(S)-7-((R)-sec-butoxy)-1-(4-chlorophenyl)-6-methoxy-2-(4-(methyl(pyridin-4-ylmethyl)amino)phenyl)-1,2-dihydroisoquinolin-3(4H)-one | C33 H34 Cl N3 O3 | 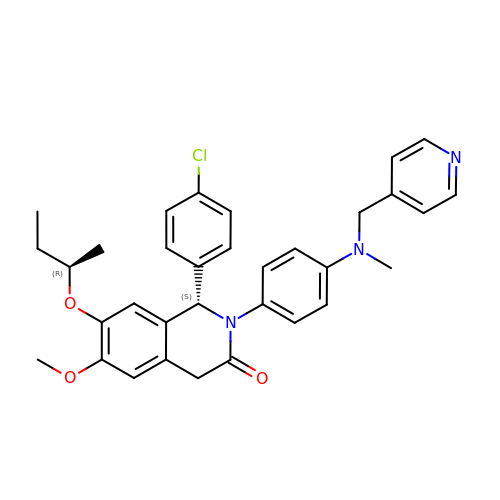RNOXGLRIZIHGIA-NBLPZQPVSA-N>MRIYVLGA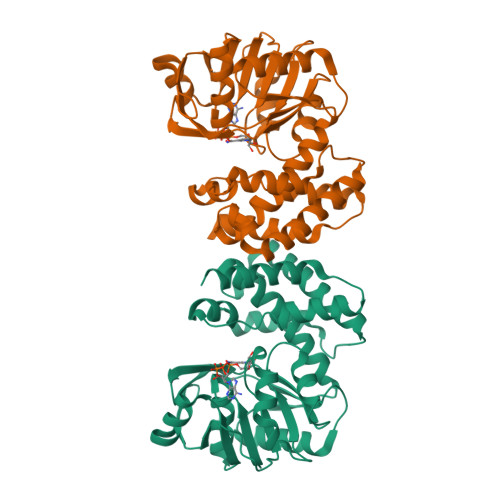GSIGSLFGALLARAGNDVTLIGRREQVDAINKNGLHVFGAEEFTVKPKATIYAPEEPPDLLILAVKSYSTKTALEAARQCIGRNTWVLSIQNGLGNEELALKYTPNVMGGVTTNGAMLVEWGKVLWAGKGITVIGRYPTGRDDFVDEVASVFNEAGIDTSVTENAIGWKWAKAIVNSVINGLGTVLEVKNGHLKDDPHLEGISVDIAREGCMVAQQLGIEFEIHPLELLWDTIERTRENYNSTLQDIWRGRETEVDYIHGKIVEYARSVGMEAPRNELLWVLVKAKERINRGKTRNISEGC[4x]>MSCPVPACCALLLVLGLCRARPRNALLLLADDGGFESGAYNNSAIATPHLDALARRSLLFRNAFTSVSSSSPSRASLLTGLPQHQNGMYGLHQDVHHFNSFDKVRSLPLLLSQAGVRTGIIGKKHVGPETVYPFDFAYTEENGSVLQVGRNITRIKLLVRKFLQTQDDRPFFLYVAFHDPHRCGHSQPQYGTFCEKFGNGESGMGRIPDWTPQAYDPLDVLVPYFVPNTPAARADLAAQYTTVGRMDQGVGLVLQELRDAGVLNDTLVIFTSDNGIPFPSGRTNLYWPGTAEPLLVSSPEHPKRWGQVSEAYVSLLDLTPTILDWFSIPYPSYAIFGSKTIHLTGRSLLPALEAEPLWATVFGSQSHHEVTMSYPMRSVQHRHFRLVHNLNFKMPFPIDQDFYVSPTFQDLLNRTTAGQPTGWYKDLRHYYYRARWELYDRSRDPHETQNLATDPRFAQLLEMLRDQLAKWQWETHDPWVCAPDGVLEEKLSPQCQPLHNELRSHHHHHH[2x]

Mucopolysaccharidosis type IIIA (MPS IIIA) is caused by the functional defect of N-sulfoglucosamine sulfohydrolase (SGSH; also known as sulfamidase, sulfamate sulfohydrolase and heparan N-sulfatase; EC 3.10.1.1) and represents one of the most frequent lysosomal storage diseases worldwide. SGSH belongs to the sulfatase family and catalyses the cleavage of N-linked sulfate groups from the GAGs heparan sulfate and heparin. The leading cysteine is post-translationally converted to a formylglycine (FGly) residue, which is crucial for the catalytic process. Despite the low sequence identity between this unique N-sulfatase and the group of O-sulfatases, they share a similar overall fold and active-site architecture, including a catalytic formylglycine, a divalent metal-binding site and a sulfate-binding site.

Here, the crystal structure of glycosylated SGSH is presented at 2 Å resolution. Two crystal forms of glycosylated SGSH were grown at different pH values. The crystal form grown at pH 7.5 is designated crystal form S (small unit cell). The structure of this form was refined to 2.00 Å resolution. There are two molecules in the asymmetric unit of crystal form S and eight molecules in that of form L. The enzyme appears to exist as a homodimer in both crystal forms. The enzyme subunits display a low rigid-body structural flexibility in the S form (Cα r.m.s.d. of 0.20 Å between the two chains, with NCS restraints) as well as the L form (r.m.s.d. ranging from 0.10 to 0.17 Å, with NCS restraints). The relative orientation of the dimer subunits in the L form differs from that in the S form by 2.6–3.0°, indicating that the dimer interface is slightly flexible, possibly owing to crystal packing. There are four cis-peptide bonds in both chains, between prolines and the preceding Gly127, Asp179, Ala482 and Ser492; all of them lie in good density. Electron density consistent with the position of a divalent metal ion in O-sulfatases was interpreted as Ca2+ based on bond-valence calculations. Difference density next to FGly70 in the active site could be modelled as a covalently bound phosphoryl group.During glycolysis, pyruvate kinase (PK) catalyzes the irreversible phosphorylation of ADP at the expense of phosphoenolpyruvate (PEP), yielding pyruvate and ATP. Previous characterization of cytoplasmic T. gondii pyruvate kinase (TgPK1), using either parasite extracts or a recombinant purified enzyme, indicated that this enzyme was allosterically activated by glucose 6-phosphate (G6P), which enhanced its activity under PEP unsaturated conditions. We solved the structure of two different constructs of TgPK1: the full-length enzyme (Met1 to Glu531 plus its N-terminal 6×His tag), which crystallized in the absence of substrates, effectors or added ions (“full TgPK1”); and an N-terminal truncated version starting at position Ile39 (“truncated TgPK1”). In both crystals, the asymmetric unit is composed of a tetramer with imperfect D2 symmetry.

The full length crystal lacked electron density for the initial 40 residues, the same ones absent in the truncated form. The monomers from the full length TgPK1 structure were all similar to each other, superposing over all atoms with rmsd values under 1 Å. A notable difference among the four monomers was the complete absence of electron density for the B domain in one of the chains (D), which has not been reported for any PK structure. Within the crystal lattice this domain was exposed to a solvent channel and the closest crystallographic neighbor is a C domain from chain C. The missing domain had little to no influence over the quality of the A domain within chain D, whose b-factors were similar to the average of the structure. First, the full length structure showed three monomers in an open inactive conformation and one subunit where there was no electron density for the B domain (disorder likely due to lack of crystal contacts). This is consistent with the B domain existing in solution as a continuum of open conformations. Additional disordered regions included several loops in the full length C domain (Val407-Pro409, Pro480-Thr485 and Lys515-Ser522). In the full length structure the differences between the A–A′ dimer interfaces are smaller when compared to the truncated TgPK1 but in both cases the smaller buried surface is associated with the outlier B domain conformation.

>MHHHHHHSSGRENLYFQGIRMSQILEPRSEEDWTAHRTRIVCTMGPACWNVDTLVKMIDAGMNVCRLNFSHGDHETHARTVQNIQEAMKQRPEARLAILLDTKGPEIRTGFLKDHKPITLQQGATLKIVTDYNLIGDETTIACSYGALPQSVKPGNTILIADGSLSVKVVEVGSDYVITQAQNTATIGERKNMNLPNVKVQLPVIGEKDKHDILNFGIPMGCNFIAASFVQSADDVRYIRGLLGPRGRHIRIIPKIENVEGLVNFDEILAEADGIMIARGDLGMEIPPEKVFLAQKMMIAKCNVVGKPVITATQMLESMIKNPRPTRAEAADVANAVLDGTDCVMLSGETANGEFPVITVETMARICYEAETCVDYPALYRAMCLAVPPPISTQEAVARAAVETAECVNAAIILALTETGQTARLIAKYRPMQPILALSASESTIKHLQVIRGVTTMQVPSFQGTDHVIRNAIVVAKERELVTEGESIVAVHGMKEEVAGSSNLLKVLTVE[4x]> MTWPLPDRLSINSLSGTPAVDLSSFTDFLRRQAPELLPASISGGAPLAGGDAQLPHGTTIVALKYPGGVVMAGDRRSTQGNMISGRDVRKVYITDDYTATGIAGTAAVAVEFARLYAVELEHYEKLEGVPLTFAGKINRLAIMVRGNLAAAMQGLLALPLLAGYDIHASDPQSAGRIVSFDAAGGWNIEEEGYQAVGSGSLFAKSS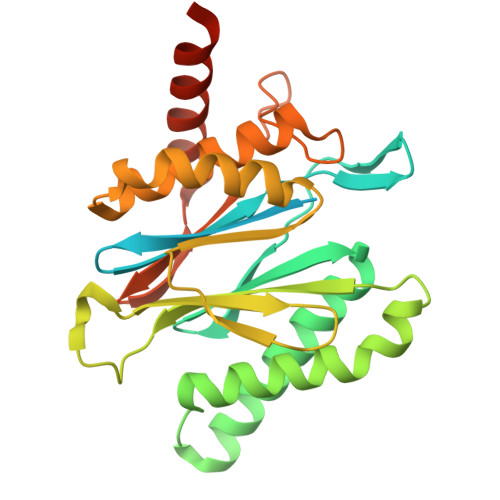MKKLYSQVTDGDSGLRVAVEALYDAADDDSATGGPDLVRGIFPTAVIIDADGAVDVPESRIAELARAIIESRSGADTFGSDGGEK> MAHHHHHHMRITVDRSQFFKSLGRVHRVVERRNTVPILSNVLIDAENGSVQLKATDLDLEVTESFTVNIEKAGAITVPAYLLYDIVRKLPDGSEIVLSVDENQASAMSIVSGCTHFQLQCLPKIDFPESLPGQFGCRFFLSASKLKHLLDCTQFAISTEETRYYLNGIYFHIVHDDVLKLRLVATDGHRLAQVDMEAPSGVDGMPGVIIPRKAVGELQKLLSEEIDGDVCIELSETKIRFSLGSVVFTSKLVDGTFPDYQR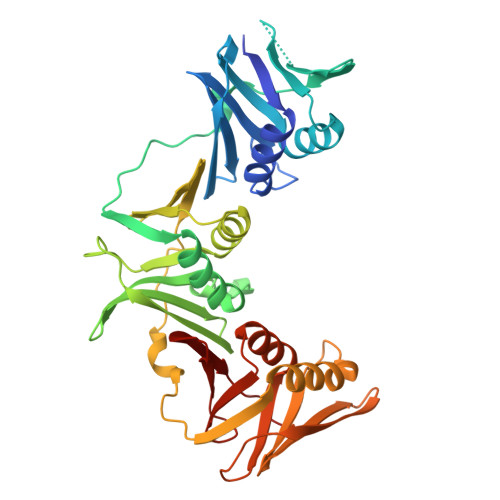VIPLGNDRKLIVNRQDFSSAVDRVSTISNDRGRAVKLTIEHGQLKLVVNNPDSGSAEDQLAATYTSEPLEIGFNSRYLLDIAGQLSSDEMVFMLSDAVAPALIRDNNNAEVLYVLMPVRV> SGLDKYLPGIEKLRRGDGEVEVKSLAGKLVFFYFSASWCPPCRGFTPQLIEFYDKFHESKNFEVVFCTWDEEEDGFAGYFAKMPWLAVPFAQSEAVQKLSKHFNVESIPTLIGVDADSGDVVTTRARATLVKDPEGEQFPW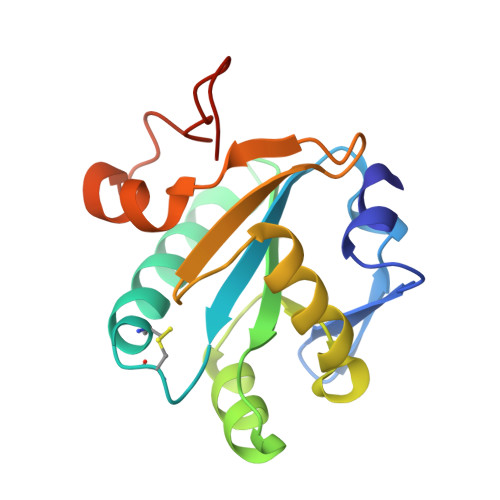KDAPLEHHHHHH> SDRLNAGKSLGAGGSLAEGPYLFIMQNDCNLVLYDNNRAVWASGTNGKASNCILKMQRDGNLVIYSGSRAMWASNTNRQDGNYYLILQRDRNVVIYDNSNN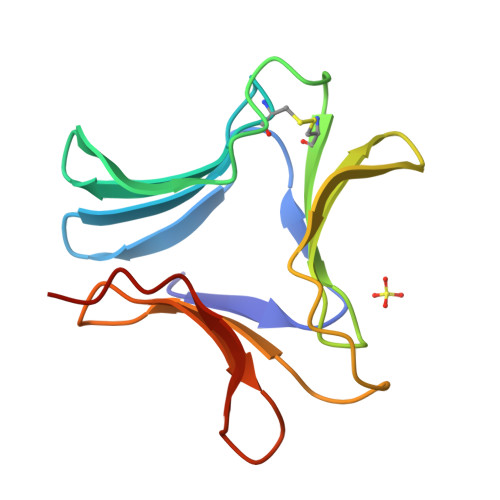AIWASGTNVGN>AQDMVSPPPPIADEPLTVNTGIYLIECYSLDDKAETFKVNAFLSLSWKDRRLAFDPVRSGVRVKTYEPEAIWIPEIRFVNVENARDADVVDISVSPDGTVQYLERFSARVLSPLDGRRTESDSQT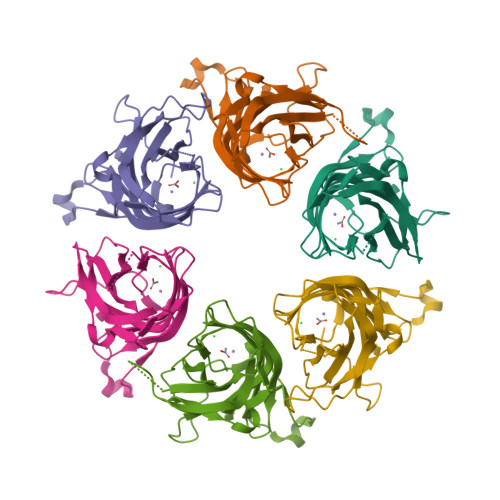LHIYLIVRSVDTRNIVLAVDLEKVGKNDDVFLTGWDIESFTAVVKPANFALEDRLESKLDYQLRISRQGGHHHHHH[6x]>[2x]ELLEGELKTAALAQHDEAMGGSLRRKGESVKKRLVSGTAASLQELSLQPSSNGIASAGKSEDGEAGDGMSGEFGAALTDSNVENNVKAFDLIFTKLKSTNQLERVAASYELKSCLISLAREVSTEYFQRFSNDINNKVFELIHGTDSNEKLGGVLAVDTLIDFYSHTDELPNQTSRLANYLRVLIPSNDIEVMRAAATTLGKLAVPGGTLTSEFVEFEVKTCIEWLTTSPESSSSNSKQEYRKHASLLIISSIAHNSPYLLYPFVNSILDNIWRALRDTKLVIRTDAAVTLGKCLTIINDRDSSLTKKWVQRLFNGCIYGLQLNTTVSIHGTLLVYRQLVSLEGGYLKDKYEEIYETTMKHRDNKNIIIRKEIYAIIPVLAAFDPKLFTQKYLDATMIHYLTLLKNMTSHQIALSDKGPILVSIGDIAYHVGSEIGPYLDAIVENLRDGLETKFKTRKEFEKDIFYCVSKLACAVRPLLAKYLNRGLLDALLACPLSDHMQETLLVICEKIPSMEVTVNEKLLNIICL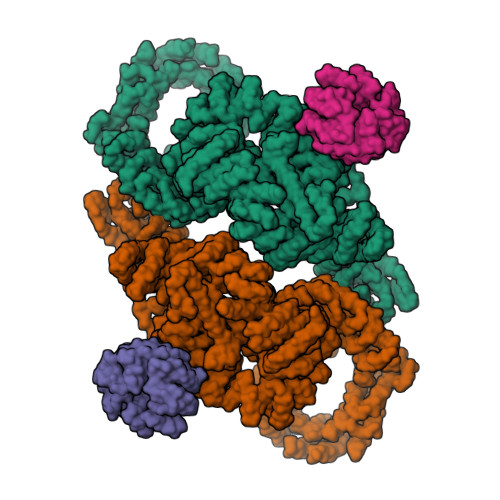VLSGEKFRPPGSPTPMKSLSSETARAYRDQSLLRKTGENNNDTLDAMILRKALRMLSDIKPKYSLTEFIRRVIISYMEHDNMQVRKLAALTSCDLFVKDSICKQTSLYALNVVSEVLSKLLTVAITDPVAEIRLEILKHLDRNFDPQLSQPDNTKLLFMALNDEVFAIQMEAMKICGRLALVNPAYVIPSLRKTLIQLLTELKHSKMTRKKEECASLLCTLISSSSDVTKPYLEPVIEILLPKSQDPSSAVASTALKALGEISVVGGEDMLPFLDELMPLIIDTFQDQSNSFKRGAALKALGQLAASSGYVIDPLLDYPELLGVLINILKSESSQNIRRETVRLIGILGALDPYKHREVERTSITNITSEQNAPPIDVALLMQGMSPSNEEYYPTVVIGVLMKILKDPSLSIHHSTVIQAIMHIFQTMGLRCVIFLKQIIPGFILVMHTCPPSLLELYFQQLSVLISIVKQHIRPHVTEIVDVISEFFPVLKLQLTIISVIESLSRALEGEFNPHLPTILSLFLDVLEKDQSNKKVVSVRILKSLVVFGPHLEEYVHLVLPTIIKLSEFSSGNLKKAAIITIGRLSKNVNALEMSSRIVQALVRVLNTSETEYVKATMNTLSLLLLQLNIDFTVFIPVINKTLVKQNIQHTIYDRLVAKLLNNEPLPTKIIIDKDFDLPNKEMDDVKVASKKLPVNQMVLKNAWDCSQQRTKEDWQEWIRRLSISLLKESSSHALRACSGLAGIYYPLARELFNASFASCWGELYTQYQEDLIQSLCAALSSPNNPPEIHQTLLNLVEFMEHDDKPLPISISTLGEYAQRCHAYAKALHYKELEFIEEPSTSTIESLITINNQLHQTDAAIGILKHAQQHHDLQLKETWYEKLQRWDDALNAYNKREAAGEDSVEVTIGKMRSLHALGEWDQLSELAADKWASSQLEVKRAIAPLAAGAAWGLAQWDRVEQYIEVMKPQSPDKAFFDAILCLHRNNFEKAAEHIFSARDLLVTEMSALVNESYNRAYGVVVRTQMVAELEEIIQYKKLPQGSERRAMIRKTWNKRLLGCQKNVDVWQRVLKVRSLVIKPKQDMKVWIKFANLCRKSGRLGLAQKTLNTLLEESGDPKNPNTARAPPPVVYAQLKYMWATGSQKEALNHLISFTSRMAHDLGLDPSNMIAQSVPQNSSVSQHHIEDYTKLLARCFLKQGEWRVSLQPNWRLENPDAILGSYLLATHFDKTWYKAWHNWALANFEVTSSLTQRIKDDKVPPTLEDASTEFTNGAVAGLNANDNFPPELVQRHVVPAIKGFFHSIALSQSSSLQDTLRLLTLWFKFGGIPEAAQAMHEGFGLIKIDNWLEVIPQLISRIHQPNQTVSRSLLSLLADLGKAHPQALVYPLTVAIKSDSVSRQRAALSIIDKMRMHSPKLVNQAELVSDELIRVAVLWHELWYEGLEDASRQFFGEHNTEKMFATLEPLHEMLKRGPETLREISFQNSFGRDLNDAYEWVLNYKRTKDINNLNQAWDIYYNVFRRISRKLPQLQTLDLQHVSPKLSAAKDLELAVPGTYHAGKPIVRITHFEPVFTVISSKQRPRRVIIKGSDGKDYQYLLKSHEDIRQDNLVMQLFGLVNTLLQNDPESFQRHLNIQQYPAIPLSPKTGLLGWVPNSDTFHVLIREHREASKIPLNIEHRIMLQMAPDYDNLTLLQKVEVFTYALDNTKGQDLYKVLWLKSRSSESWLDRRTTYTRSLAVMSMVGYILGLGDRHPSNLMLDRITGKVVHIDFGDCFEAAILREKYPEKVPFRLTRMLTYAMEVSGIEGSFRITCENVMMVLRDNKESLMAILEAFAYDPLINWGFDLPTHAVMEQTGIDLPLANPSELLRKGVISVEDAAKMELQQKAEVRNARATLVLKRIADKLTGNDFPRCQELSVPDQVDKLIQQATSVENLCQHYIGWCSFW;>[2x]MSVILASAGYDHTIRFWEALTGVCSRTIQHADSQVNRLEITSDKKYLAAAGHLHVRLYDIRSNNPNPVSSFEGHKGNVTSIAFQQENRWMVSSSEDGTIKVWDVRSPSVQRNYKHNAPVNEVAIHPNQGELISCDQDGNIRIWDLGENQCTNQLTPEDNTPLQSLSVASDGSMLVAGNNKGNCYVWRMPHHTDASTLEPVTKFKSHTKYITRVLLSADVKNLATCSADHTARVWNIEDNYQLETTLDGHQRWVWDCAFSADSAYLVTACSDHYVRLWDLSTSEIVRQYGGHHKGAVCVALNDV>[4x]HHHHHHLPNITILATGGTIAGGGDSATKSSYTVGKVGVENLVNAVPQLKDIANVKGEQVVNIGSQDMNDNVWLTLAKKINTDCDKTDGFVITHGTDTMEETAYFLDLTVKCDKPVVMVGAMRPSTSMSADGPFNLYNAVVTAADKASANRGVLVVMNDTVLDGRDVTKTNTTDVATFKSVNYGPLGYIHNGKIDYQRTPARKHTSDTPFDVSKLNELPKVGIVYNYANASDLPAKALVDAGYDGIVSAGVGNGNLYKSVFDTLATAAKTGTAVVRSSRVPTGATTQDAEVDDAKYGFVASGTLNPQKARVLLQLALTQTKDPQQIQQIFNQY

Bacterial L-asparaginases are amidohydrolases (EC 3.5.1.1) capable of deaminating L-asparagine and, with reduced efficiency, L-glutamine. Bacterial L-asparaginases are homotetrameric proteins of 140–150 kDa. Each subunit is built-up by nearly 330 amino acids and consists of two α/β domains connected by a ca 21 amino-acid-long random coil. To obtain high-quality crystals, we took advantage of the highly stable N24S L-asparaginase, which shares identical catalytic and structural properties with the wild-type enzyme, but has largely improved stability and forms highly ordered crystals.

The ASU of the N24S–GLU complex, solved at 1.90 Å resolution, was similar to the one of apo-N24S: it comprised the 4 A, B, C, and D monomers, with chains A/C and B/D forming the two independent intimate dimers and the biological unit rebuilt using the crystallographic C2 symmetry operators. Even here, none of the protomers in the ASU contained a complete electron density trace for the ASFL. All the active sites contained clear electron density for the L-GLU ligand. Positions of L-GLU atoms were superposable for all protomers except protomer B, in which the L-GLU Cβ was 1.7 Å shifted with respect to the corresponding atom of the other ligands. In the case of our structure, in all four N24S–GLU protomers, the oxygen atoms of the Cα carboxylic group of L-GLU are, in fact, located in the positions normally occupied by waters W1 and W2 in the apo-N24S structure. However, because of the extra CH2 group (Cγ) in its side chain compared to the one of L-ASP, the O atoms of the Cδ carboxylic group of L-GLU do not coincide either with the position of the apo-N24S W3 and W4 nor of the L-ASP Cγ carboxylic group O atoms. As a consequence of the steric hindrance induced by L-GLU “misplacement” in the binding pocket, the catalytic residues T12, Q63 and E283 are shifted from the position usually observed in both the apo- and N24S–ASP structures (respectively). Additionally, w II, which is involved in the second step of the catalysis that resolves the enzyme tetrahedral and releases the deaminated product, is absent in three of the four protomers, being present only in protomer B, where L-GLU has a conformation more similar to L-ASP. In the structure of N24S–GLU protomer D, in which the ASFL is in a conformation compatible with its closed position, the placement of L-GLU inside the binding pocket causes the shifting of catalytically relevant residues from their canonical position, causing an altered chemical geometry in the catalytic center that, in turn, can explain the less efficient catalysis. According to the collected data, the ASFL closure is less efficient in the presence of L-GLU, very likely because of the steric hindrance deriving from the extra methyl group of the side chain compared to L-ASP.> QPIFLNVLEAIEPGVVCAGHDNNQPDSFAALLSSLNELGERQLVHVVKWAKALP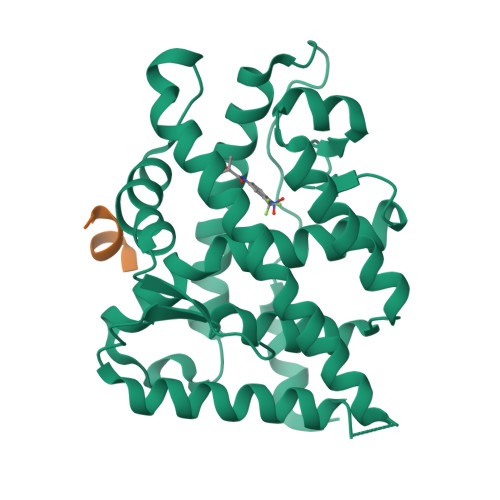GFRNLHVDDQMAVIQYSWMGLMVFAMGWRSFTNVNSAMLYFAPDLVFNEYRMHKSRMYSQCVRMRHLSQEFGWLQITPQEFLCMKALLLFSIIPVDGLKNQKFFDELRMNYIKELDRIIACKRKNPTSCSRRFYQLTKLLDSVQPIARELHQFAFDLLIKSHMVSVDFPEMMAEIISVQVPKILSGKVKPIYFHTQ;> ANSSFRDWYTSS> GHMAENREPRGAVEAELDPVEYTLRKRLPSRLPRRPNDIYVNMKTDFKAQLARCQKLLDGGARGQNACSEIYIHGLGLAINRAINI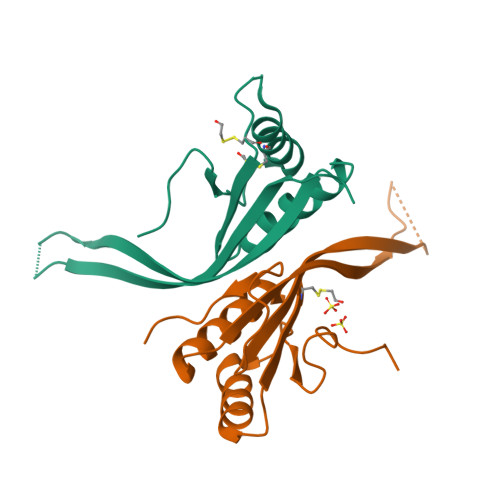ALQLQAGSFGSLQVAANTSTVELVDELEPETDTREPLTRIRNNSAIHIRVFRVTPK;> GHMENFRKVRSEEAPAGCGAEGGGPGSGPFADLAPGAVHMRVKEGSKIRNLMAFATASMAQPATRAIVFSGCGRATTKTVTCAEILKRRLAGLHQVTRLRYRSVREVWQSLPPGPTQGQTPGEPAASLSVLKNVPGLAILLSKDALDPRQPGYQPPNPHPGPSSPPAAPASKRSLGEPAAGEGSAKRSQPEPGVADEDQTA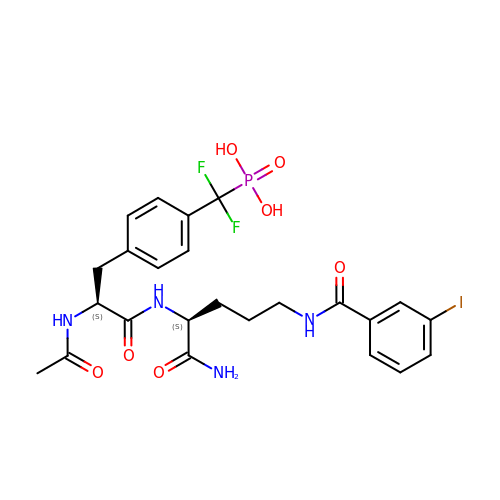N-acetyl-4-[difluoro(phosphono)methyl]-L-phenylalanyl-N~5~-(3-iodobenzoyl)-L-ornithinamide | C24 H28 F2 I N4 O7 P | DSHZHFAULLMSCZ-PMACEKPBSA-N>NDHIHRVPALTEEEIDSVAIKTFERYALPSSSSVKRKGKGVTILWFRNDLRVLDNDALYKAWSSSDTILPVYCLDPRLFHTTHFFNFPKTGALRGGFLMECLVDLRKNLMKRGLNLLIRSGKPEEILPSLAKDFGARTVFAHKETCSEEVDV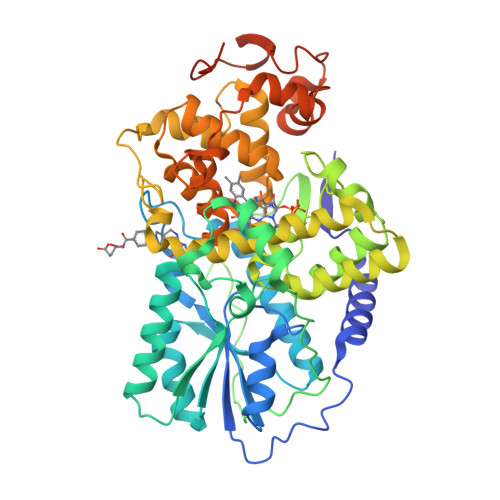ERLVNQGLKRVGNSTKLELIWGSTMYHKDDLPFDVFDLPDVYTQFRKSVEAKCSIRSSTRIPLSLGPTPSVDDWGDVPTLEKLGVEPQEVTRGMRFVGGESAGVGRVFEYFWKKDLLKVYKETRNGMLGPDYSTKFSPWLAFGCISPRFIYEEVQRYEKERVANNSTYWVLFELIWRDYFRFLSIKCGNSLFHLGGPRNVQGKWSQDQKLFESWRDAKTGYPLIDANMKELSTTGFMSNRGRQIVCSFLVRDMGLDWRMGAEWFETCLLDYDPCSNYGNWTYGAGVGNDPREDRYFSIPKQAQNYDPEGEYVAFWLQQLRRLPKEKRHWPGRLMYMDTVVPLKHGNGPMAGGSKSGGGFRGSHSGRRSRHNGP[2x]> DSDDRVTPPAEPLDRMPDPYRPSYGRAETVVNNYIRKWQQVYSHRDGRKQQMTEEQREWLSYGCVGVTWVNSGQYPTNRLAFASFDEDRFKNELKNGRPRSGETRAEFEGRVAKESFDEEKGFQRAREVASVMNRALENAHDESAYL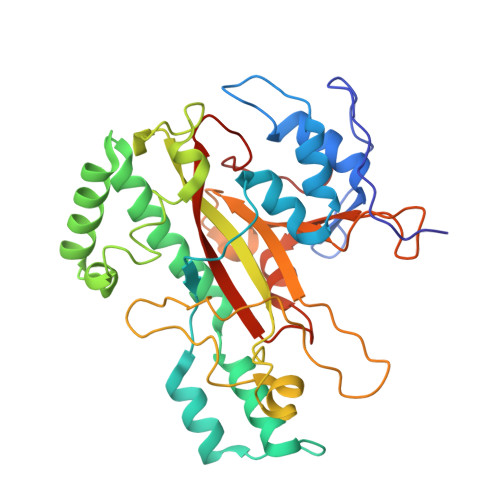DNLKKELANGNDALRNEDARSPFYSALRNTPSFKERNGGNHDPSRMKAVIYSKHFWSGQDRSSSADKRKYGDPDAFRPAPGTGLVDMSRDRNIPRSPTSPGEGFVNFDYGWFGAQTEADADKTVWTHGNHYHAPNGSLGAMHVYESKFRNWSEGYSDFDRGAYVITFIPKSWNTAPDKVKQGWP> QYSPNTQQGRTSIVHLFEWRWVDIALECERYLAPKGFGGVQVSPPNENVAIYNPFRPWWERYQPVSYKLCTRSGNEDEFRNMVTRCNNVGVRIYVDAVINHMCGNAVSAGTSSTCGSYFNPGSRDFPAVPYSGWDFNDGKCKTGSGDIENYNDATQVRDCRLTGLLDLALEKDYVRSKIAEYMNHLIDIGVAGFRLDASKHMWPGDIKAILDKLHNLNSNWFPAGSKPFIYQEVIDLGGEPIKSSDYFGNGRVTEFKYGAKLGTVIRKWNGEKMSYLKNWGEGWGFVPSDRALVFVDSHDNQRGHGAGGASILTFWDARLY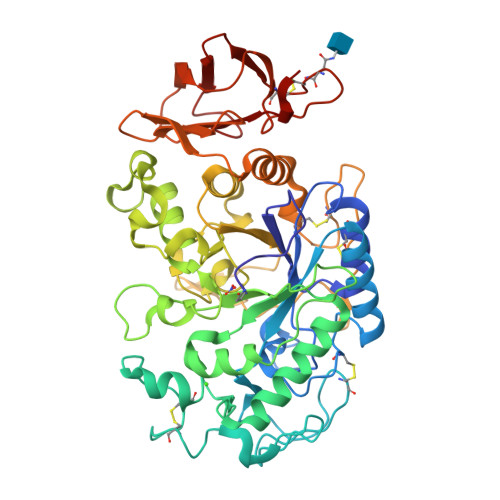KMAVGFMLAHPYGFTRVMSSYRWPRQFQNGNDVNDWVGPPNNNGVIKEVTINPDTTCGNDWVCEHRWRQIRNMVIFRNVVDGQPFTNWYDNGSNQVAFGRGNRGFIVFNNDDWSFSLTLQTGLPAGTYCDVISGDKINGNCTGIKIYVSDDGKAHFSISNSAEDPFIAIHAESKL> MASPALQTCWRNLARLSGAQVRPSHFGAFSLGSRMSPFSSLLGARASPIATGRAGLRFLSSAAPNPGKKPASAAPPAGTNHGRITQVIGAVVDVHFDEQLPPILNSLEVQGHTNRLVLEVAQHLGENTVRTIAMDATEGLVRGQKVVDTGAPIQVPVGVETLGRIMNVIGEPVDECGPVPAKKTYSIHRAAPLFADQSTEPGLLQTGIKVVDLLAPYAKGGKIGLFGGAGVGK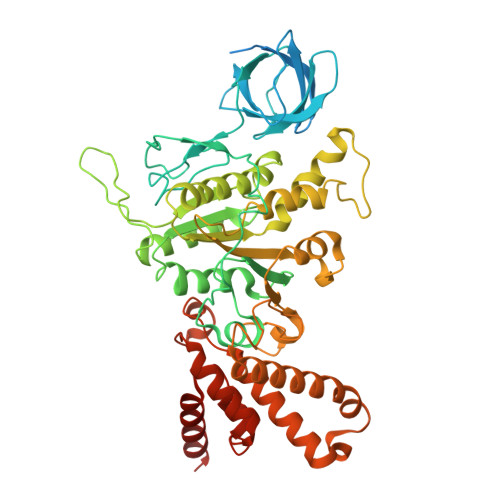TVLIMELINNVANKHGGFSVFAGVGERTREGNDLYHEMMTTGVIKRKKLEDGKFDFTGSKAALVYGQMNEPPGARARVALTALSVAEYFRDEQGQDVLLFIDNIYRFTQAGSEVSALLGRIPSAVGYQPTLATDLGQLQERITTTKKGSITSVQAVYVPADDLTDPAPATTFAHLDATTVLSRQIAELGIYPAVDPLDSTSRMLAPEIVGQEHYDTARATQKLLQDYKSLQDIIAILGMDELSEEDKLVVSRARKIQRFLSQPFTVAEVFTGKPGRFVELPETIKSAQTILRGECDDLPEMAFYMCGGLEEVRSKAVKMAQEAASGK> GPAPARFCVYYDGHLPATRVLLMYVRIGTTATITARGHEFEVEAKDQNCKVILTNGKQAPDWLAAEP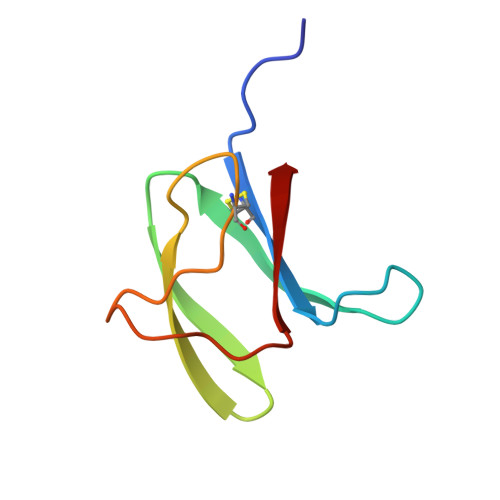Y> VEPI;> VVGGTEAQRNSWPSQISLQYRSGSSWAHTCGGTLIRQNWVMTAAHCVDRELTFRVVVGEHNLNQNNGTEQYVGVQKIVVHPYWNTDDVAAGYDIALLRLAQSVTLNSYVQLGVLPRAGTILRNNSPCYITGWGLTRTNGQLAQTLQQAYLPTVDYAICSSSSYWGSTVKNSMVCAGGDGVRSGCQGDSGGPLHCLVNGQYAVHGVTSFVSRLGCNVTRK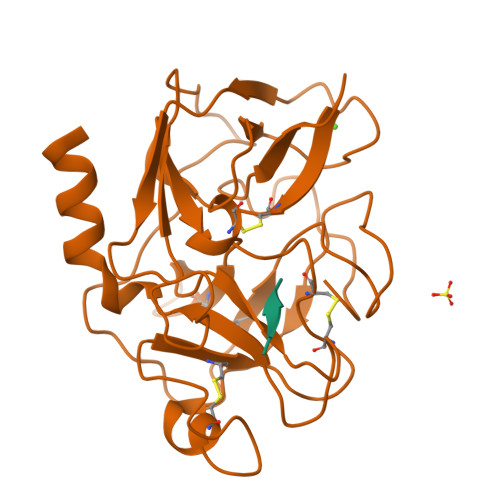PTVFTRVSAYISWINNVIASN>MRSRRVDVMDVMNRLILAMDLMNRDDALRVTGEVREYIDTVKIGYPLVLSEGMDIIAEFRKRFGCRIIADFKVADIPETNEKICRATFKAGADAIIVHGFPGADSVRACLNVAEEMGREVFLLTEMSHPGAEMFIQGAADEIARMGVDLGVKNYVGPSTRPERLSRLREIIGQDSFLIS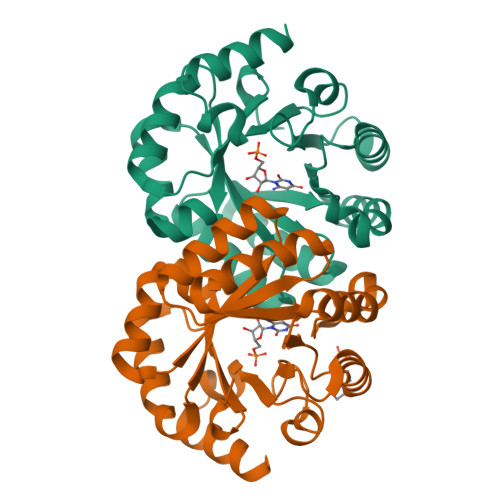PGVGAQGGDPGETLRFADAIIVGRSIYLADNPAAAAAGIIESIKDLLIPEDPAANKARKEAELAAATA[2x]> MSRLIFEHQRRLTPPTTRKGTITIEPPPQLPRVVPPSLLRRVLPFLIVILIVGMIVALFATGMRLISPTMLFFPFVLLLAATALYRGGDNKMRTEEVDAERADYLRYLSVVRDNVRAHAAEQRAALEWSHPEPEVLATIPGTRRQWERDPRDRDFLVLRAGRHDVPLDAALKVKDTADEIDLEPVAHSALRGLLDVQRTVRDAPTGLDVAKLARITVIGEADEARAAIRAWIAQAVTWHDPTMLGVALAAPDLESGDWSWLKWLPHVDVPNEADGVGPARYLTTSTAELRERLAPALADRPLFPAESGAALKHLLVVLDDPDADPDDIARKPGLTGVTVIHRTTELPNREQYPDPERPILRVADGR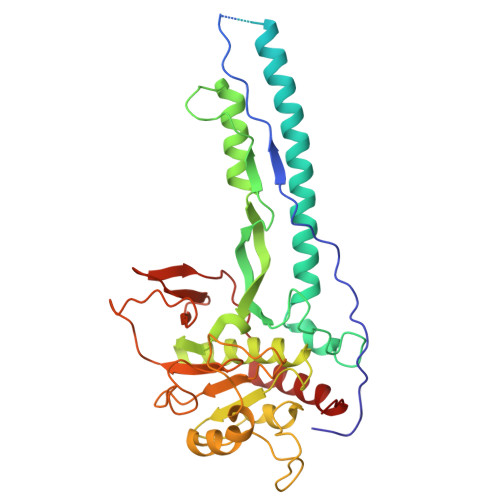IERWQVGGWQPCVDVADAMSAAEAAHIARRLSRWDSN> MAEYFTYSKKRKEFNNPINFQDTETRYGGIQNQVVNINQYVQRNPNFIDLDNIAELSEHSVNTERVKTGDRGMSHKEGGWPGNVDPNEAQETGRFKKRIEKDTSFPQAVKDLKEGVEKCIYQNNQIDLLEEYFEGETSEHVVENLSSKTLMLFKDEKEICKRSVSEISWHPEGPTKVAVSYAIMRFQQMPEKMPTQAYVWDLLNPNSPEIKLMSPSAVTNISYNQKIPDQIGGGCYNGLLAVWDGRKGENPIMISPVENSHYEPVTHFHWLMSKTGSECVTTSTDGKVMWWDTRKFEAGPVEKLNIIEGLGENEEIIGGTALEYNVEAGPSKFLIGTESGSILTANKKLKKPVEITTRYGLDQGRHLGPVYSINRSNQNPKYFLSVGDWSCKIWVEDLKTPIIRTKYHGSYLSDGCWSPTRSGAFFLVRRDGWMDVWDYYYRQNEIAFSHKVSDSPLTCIKINQTGGAYHNSGKLCAIGDQDGTVTILELCDSLYTMQPKEKDIINEMFEREYRKEKNLETIKKQQELAKRQVQKDMGSQKEKWEKKKLEMIETAEASFHENLAKNPVNEEEFNELDSPSEKRKKTNQNQGREQEEQSREEQEASGNFNQQQQQQQEEEQQQE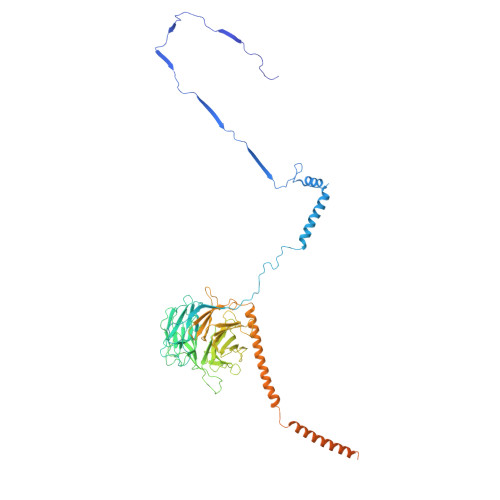GEQQHHQNQEHQNGQGHENGQEEGEENGEEGNQQENEGQEENEQQQE>TPQNITDLCAEYHNTQIHTLNDKIFSYTESLAGKREMAIITFKNGATFQVEVPGSQHIDSQKKAIERMKDTLRIAYLTEA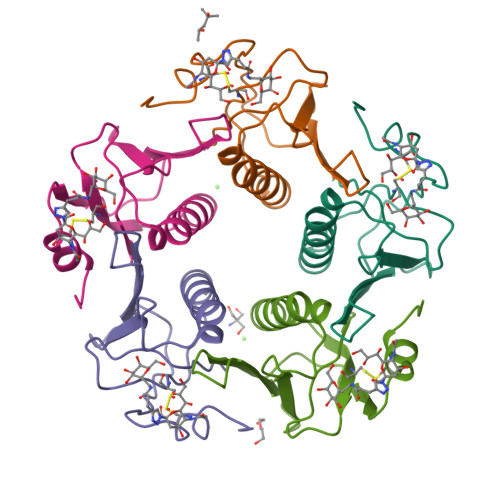KVEKLCVWNNKTPHAIAAISMAN[5x]>[3x]GPLGSPEFPRRGKPEAQPFAHLTINAASIPSGSHKVTLSSWYHDRGWAKISNMTLSNGKLRVNQDGFYYLYANICFRHHETSGSVPTDYLQLMVYVVKTSIK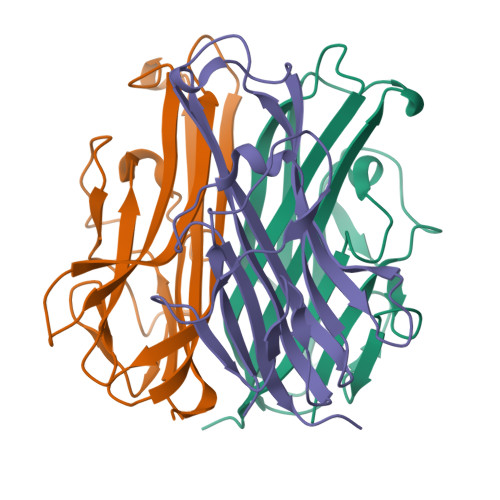IPSSHNLMKGGSTKNWSGNSEFHFYSINVGGFFKLRAGEEISIQVSNPSLLDPDQDATYFGAFKVQDID ethyl (~{Z})-3-[1-[(~{E},1~{R},4~{R})-4-[(1~{R},3~{a}~{S},4~{E},7~{a}~{R})-7~{a}-methyl-4-[(2~{Z})-2-[(3~{S},5~{R})-2-methylidene-3,5-bis(oxidanyl)cyclohexylidene]ethylidene]-2,3,3~{a},5,6,7-hexahydro-1~{H}-inden-1-yl]-1-oxidanyl-pent-2-enyl]cyclopropyl]prop-2-enoate 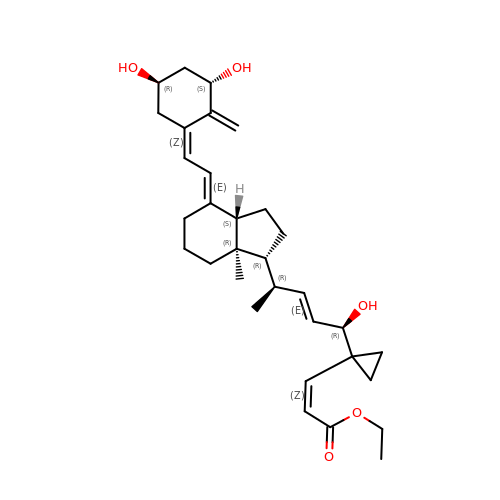| C32 H46 O5 | FUDAEUIGIJZUAY-MRFCKDSNSA-N> MKHLPSENAAPMAVGIQFSVGLSALGCELNQIKQALQQPQQTLSLRDDLIADRDVWVGQYTHPLCSSVPDAMRSVDSRNLRFALTALSKIETELKAYTASFENKRLAIVVGTSTSGIADNELLLKQYFQGQTDLSISHYPQEMSCLAKALQQYLGWEGPAYTISTACSSSAKALAAGQRLLHADLADVVLVGGVDTLCKLTLNGFNSLESLSAHICQPCGISRDGINIGEAAAFFVLSKEQAPVMLMGAGETMDAWHISAPHPEGKGAALAMQRALDMAHISAQEVGYINLHGTATPQNDAMEIKAVRQVFGVYQVALSSTKHKTGHCLGAAGAIEAFICEQVLKDQSWLPLHQNVEIDPDLVDQNYVQEAELTQPIR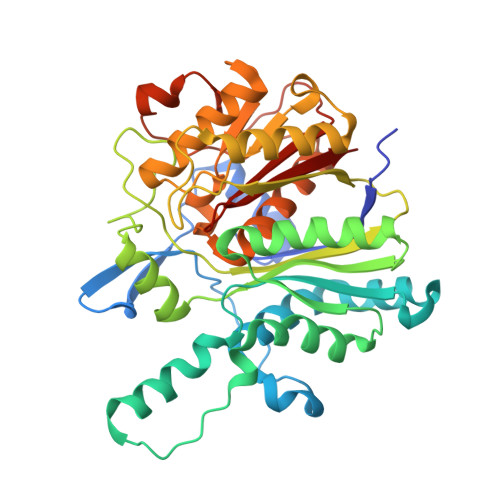YVMSNSFAFGGSNISLVFGVKP In the archaeon Sulfolobus acidocaldarius, the GTPase Saci1281 (from hereon: SaGPN) represents the solitary GPN-loop GTPase. Structural analysis of the GTP- and GDP-bound states of the Sulfolobus acidocaldarius GPN enzyme (SaGPN) showed that this central GPN-loop GTPase adopts two distinct quaternary structures. The general structure of SaGPN involves 12 α-helices and a five-stranded, parallel β-sheet that is sandwiched by α6/α8 and α1/α12, respectively. The dimer interface emerges alongside the surface of helices α3, α5, α8, and α11, whereby α8 contributes substantially to the dimeric assembly due to its central position allowing the formation of a hydrophobic pocket.

The GDP-bound structure contains three molecules per a.s.u., where monomers A and C form together a physiological dimer. Likewise, monomer B forms a dimer with its crystal mate B′. The difference between both SaGPN dimers in this crystal form is minor, as a superposition of the dimers yields an r.m.s.d value of only 0.24 Å (445 Cα atoms). In monomers A and B, a double hydrogen bond between N70 of the GPN motif with Q106′ is formed, whereas altered χ2 angles of N70′ and Q106 of monomers C and A, respectively, are consistent only with the formation of a single H-bond. Apart from the missing γ-phosphate the binding mode of Mg2+·GDP to SaGPN is comparable to that of Mg2+·GppNHp. Interestingly, we observe a water molecule coordinated between D38 and N70′ (primed residues mark the second protomer) close to the position observed before for the inline attacking water molecule of the GppNHp-bound state thus corroborating the role of N70′ of the GPN motif in positioning the water molecule for catalysis. However, due to the loss of the γ-phosphate interaction, the GPN loop detaches from the nucleotide, resulting in an opened substrate pocket around the phosphates. Additionally, the γ-phosphate-GPN interaction is lost after hydrolysis, resulting in a swivel-off motion of the GPN-loop including the preceding α2 skids (residues V58-Y65), thus relaxing the whole assembly. After GTP hydrolysis and loss of the γ-phosphate, the substrate pocket switches from a closed into an open state by losing the interaction to the second protomer’s GPN motif. Accordingly, the GDP-bound state of SaGPN apparently represents a conformation, whose stability exceeds those of the non-covalently linked GDP·AlF4−- or GDP·Pi-bound states.

>[3x]MHHHHHHHHHHLEVLFQGPSYFIFVLGTAGSGKTTLVKALQDYLLNNELDTAIINLDPAVEVLPYKPDIDAREYVDVYDVMNKYELGPNSSLVISVDLLLTKAKELKEDLNQLQANYVLVDTPGQIELFAYRDTGKILSSFISEGSKSVSVFLFDSYLSKDPKSFLSLFLLSSSIKFRIDMPQISVLSKVDLLSSSELERMRSWIEDGSIIDELGSIDEYSFELVKTIVENLESFPIPVSSTNFSGLDQLYAEVQKVLAGGEDFETEEPNPRLA> LAAALEGPYPVEEIRLPRAGGPLGLSIVGGSDHSSHPFGVQEPGVFISKVLPRGLAARSGLRVGDRI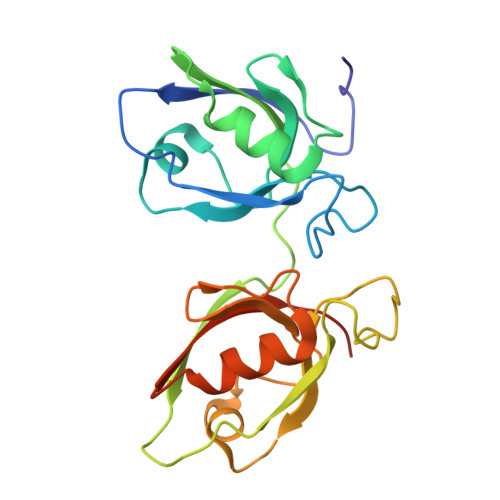LAVNGQDVRDATHQEAVSALLRPCLELSLLVRRDPAPPGLRELCIQKAPGERLGISIRGGARGHAGNPRDPTDEGIFISKVSPTGAAGRDGRLRVGLRLLEVNQQSLLGLTHGEAVQLLRSVGDTLTVLVCDGFEASTDAALEVS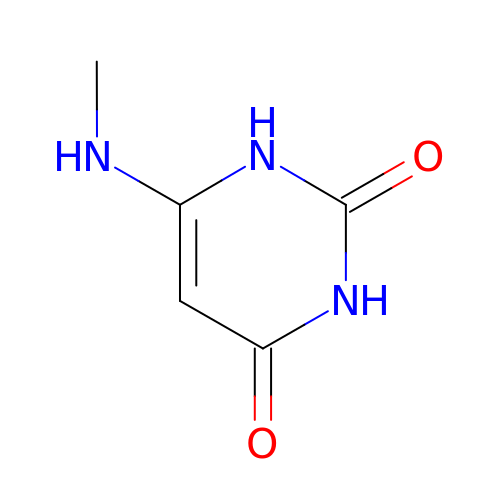6-(METHYLAMINO)-1H-PYRIMIDINE-2,4-DIONE | C5 H7 N3 O2 | ISUVRRPGXQIRDM-UHFFFAOYSA-N> MAGQEDPVQREIHQDWANREYIEIITSSIKKIADFLNSFDMSCRSRLATLNEKLTA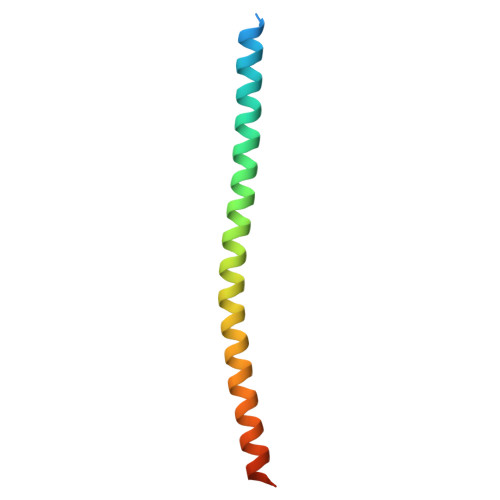LERRIEYIEARVTKGETLT>[4x]VIPDYFKQSFPEGYSWERSMTYEDGGICIATND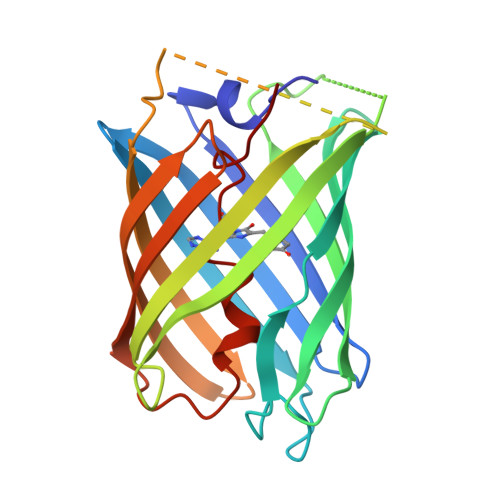ITMEGDSFINKIHFKGTNFPPNGPVMQKRTVGWEASTEKMYERDGVLKGDVKMKLLLKGGGHYRCDYRTTYKVKQKPVKLPDYHFVDHRIEILSHDKDYNKVKLYEHAVARNSTDSMDELYKGGSGGMVSKGEETITSVIKPDMKNKLRMEGNVNGHAFVIEGEGSGKPFEGIQTIDLEVKEGAPLPFAYDILTTAFHYGNRVFTKYPR> MDGSRGTAPGGDDLRGDRRDSYQGEDREDSHLLGALEDGNHQQSQGHGGGSGFYHHNVNSSSASVLEGVEMAHDELFAGPVAESVPTSVSAFSHRHGRAESVASFSFYHEQDDQREELEAPPGSLGARLSIDDLDELPFEEEGLSESEMPEQLDTFGIDLEWGSMNNGYPLIRRSSTHSQFSAHHRLLRRESGVSAASGYTGGRSSQKMRLDNDDLTIAISGFITNRIGFAIYIVLCVLTGGIAWLFLRWYPKYYVKLVGCATPFRDCQWVVIEDHFNKMTILSIRVKPYNRPLSTVFGTPSRATSWPLAQDPDPVLRELRSITYCYYKFYYHPVLDKFFCCNGWKDPQWNSMQNARSGLHGDEKAHREAVFGPNSIDVDEQSILQLLVSEILTPFYAFQVFSLILWLCDEYYYYAAAILLISAGSIITSLLETKETRRRLREMSRFECEVRVFRGGFWRTFPSSDLVPGDVYEVSDPSLTQIPADSLLLTGDCIVNESMLTGESVAVSKTPATNETLAKLNPAASTFSHDVDKHFLYCGTKLIRARQRLADTDEAAAVALVVRTGFNTTRGALVRSMLVPKPSKFKFYEDSFRYLKVMGCLAGLAFIVSLVNFIRLKLHWTLILLRALDLLTIVVPPALPATLTIGTSFAVQRLKGKKIFCTSPQRVNVGGKIDLMCFDKTGTLTEEGLDVLGIRVASRVSNRFTELLTNVDDLTWSCDSVSNGDEVKPADHVDGSSLKKDKTKPLDPYRAALYVMASCHSLRIVDGVAVGDPLEVKMFEFTGWSYEEGFIAGEVISTEGRGDISPSIARPPRYMTSQEMSIGEAPPAVGVLRAFDFNPLLRRSSVIARVVGNSGGYALVKGSPECMPEICRPETLPSDFDELLSYYTHAGYRVIACATKRIPKLNLVSVNRMTRDEVESGLDFVGFIIFENKLKPTTTSVIKELLSSNIGTVMITGDNIRTAVSVARQCGIIEEHAHCYMPRFIEGNADDCNAKLRWESINNPALELDPWTLLPMPVPPQTDASLPYDVSNIRNYAIAVTGDVFRWIVDHAPTDVLHRMLVLGKVYARMSPDEKQELVKKFQSIDYSCGFCGDGANDCAALKAADVGISLSEAEASVAAPFTSQIFDIRCVPEVIREGRASLVTSFSCFKYMSLYSFIQFTSVSFLYVSASNLGDFQFLYIDLMLILPIAVFMSWAGPHSKLCAKRPVSDLVSRKVLVPLLSHVFVCVMIQALAWVAVRQQPWYIPPIVDTEKSNIENSENTTLFFASCFEYILSGVVLNAGRPFRQSPLETWPFLSAVAVTLIATLLMLLVPPYWLFEFMQLTWMSWTFKITLIAFGFVYFLIAWTGEHYLFLWLARFLGRMRQRLFKQPKQRKLYKIVKEKLVFENLYF

P-type ATPases form a large membrane protein superfamily that couples ATP hydrolysis to the transport of cargo across biological membranes. In human cells, P5B-ATPases execute the active export of physiologically important polyamines such as spermine from lysosomes to the cytosol, a function linked to a palette of disorders. Here we describe a series of cryo-electron microscopy structures of a yeast homolog of human ATP13A2-5, Ypk9, determined at resolutions reaching 3.4 Å, and depicting three separate transport cycle intermediates, including spermine-bound conformations. Ypk9 exhibits ten TM helices and a soluble N-terminal domain (NTD) in close proximity to the membrane, perhaps involved in lipid regulation.

Next, additional structures were determined, all in the presence of SPM, and using N- or C-terminally linked GFP protein. Structural analyses to SERCA and ATP11C-CDC50A suggest the SPM-structures are indeed caught in separate E2P and E2.Pi configurations, with the E2.PiSPM structure indicating the presence of cargo is sufficient to stabilize an E2.Pi state. While the E2.Pi structures are highly similar, distinctions are identified between the two recovered E2P states (see further below). Spermine uptake is accomplished through an electronegative cleft lined by transmembrane segments 2, 4 and 6. The cleft harbors an additional, elongated density compatible with the presence of SPM. Equivalently, completion of cargo-binding is linked to the proceeding E2.Pi state, where SPM is accommodated in a cavity on the luminal side, coordinated by conserved acidic and hydrophobic residues, including the conserved VPPALP motif. As such, the composition of the cavity also allows binding of shorter physiological polyamines, e.g., SPD and putrescine, in a similar manner. Comparison of the structures reveals major rearrangements of the TM helices linked to SPM uptake. Based on these observations, we speculate that the affinity for SPM increases from the E2Pinhib to the E2P* and E2.Pi states. The structural changes that orchestrate the SPM pocket are coupled to a rotation of the A-domain, leading to a 6 Å movement of the TGES dephosphorylation loop as observed in other P-type ATPases, and a similar movement of the adjacent NTD.> MSAYRHAVERMDSSDLACGVVLHSAPGYPAFPVRLATEIFQRALARLPGDGPVTLWDPCCGSGYLLTVLGLLHRRSLRQVIASD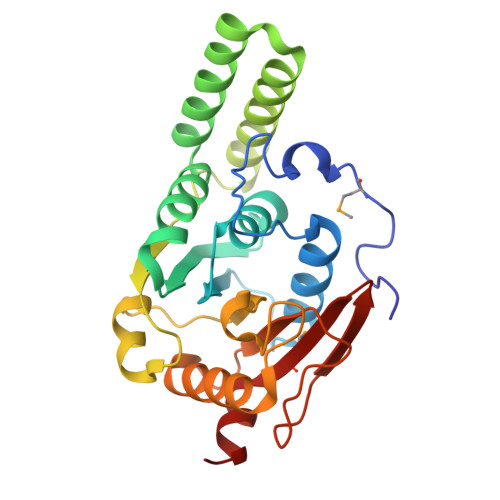VDPAPLELAAKNLALLSPAGLTARELERREQSERFGKPSYLEAAQAARRLRERLTAEGGALPCAIRTADVFDPRALSAVLAGSAPDVVLTDLPYGERTHWEGQVPGQPVAGLLRSLASALPAHAVIAVTDRSRKIPVAPVKALERLKIGTRSAVMVRAADVLEAGP> GSTGLIKHTEYMEFLKSVPTFQSLPEEILSKLADVLEETHYENGEYIIRQGARGDTFFIISKGTVNVTREDSPSEDPVFLRTLGKGDW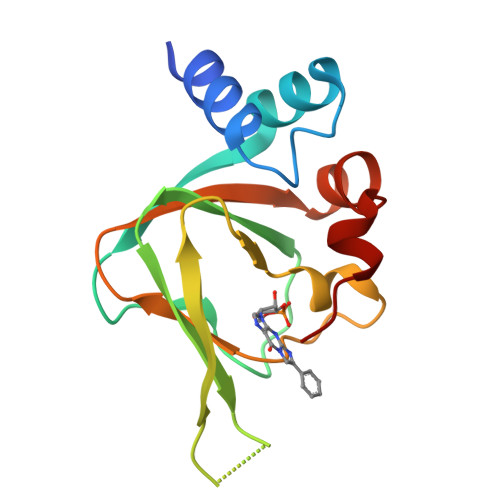FGEKALQGEDVRTANVIAAEAVTCLVIDRDSFKHLIGGLDDVSNKAY In this work, we employed an approach to disentangle noncovalent and hydrogen-bonding electric field changes during the reaction cascade of a multidomain protein, i.e., the phytochrome Agp2. Agp2 originates from Agrobacterium fabrum and carries a biliverdin (BV) chromophore. Phytochromes harbor a methine-bridged tetrapyrrole chromophore as a light-sensing unit, which upon light absorption undergoes a photoisomerization at the terminal methine bridge followed by a cascade of structural relaxations.18−21 This reaction sequence interconverts the parent states Pr and Pfr and involves proton translocation, which has been shown to be a prerequisite for the functional secondary structure transition of the tongue, a phytochrome-specific peptide segment. In the present work, we have generated two further variants with ortho-cyanophenylalanine (oCNF) at positions 165 or 192.

We determined the crystal structures of the Pfr state of Y165oCNF and F192oCNF variants with 1.90 and 2.06 Å resolution, respectively. Structural details of the ZZEssa chromophore geometry and rotamer positions of amino acids within the CBP display a very high similarity between the oCNF variants and the WT protein, whereby F192oCNF is virtually indistinguishable from the WT. The region between 1500 and 1700 cm–1 is dominated by the C=C stretching modes of the methine bridges between pyrrole rings, which are particularly sensitive toward geometrical changes of the tetrapyrrole skeleton.54 In the Pfr state, a nearly perfect agreement between the WT and F192oCNF spectra in this region underpins the preservation of the chromophore structure in both proteins. In the Pr-minus-Pfr difference spectrum of F192oCNF, the lack of a positive band in this region confirms the shift of the tautomeric equilibrium toward the enol form. Phe192 is located in a hydrophobic part of the CBP. Accordingly, no strong H-bonds are expected for either pCNF or oCNF at position 192, which is confirmed by the crystal structure (F192oCNF) and the structural model (F192pCNF) for the Pfr state with the exception of a H-bond in the oCNF192 backbone to Gly173. For the sake of simplicity, we may therefore classify the H-bonds of the protein-bound phenyl substituents on the basis of the EF,tot,HB values as very weak (0–15 MV/cm), weak (15–30 MV/cm), medium (30–45 MV/cm), strong (45–60 MV/cm), and very strong (>60 MV/cm). Both F192pCNF and F192oCNF reveal only very weak H-bonding interactions because this residue is located in an essentially nonpolar pocket as shown by Pfr structures. A strong field increase upon Pr formation is also found for F192pCNF and F192oCNF, which is, however, accompanied by minima in Lumi-F and Meta-F, respectively. In both Agp2 variants carrying the nitrile group at the ortho position, the noncovalent electric fields remain largely constant during the photoconversion.

>[2x]MASTDYHVDLTNCDREPIHIPGYIQPHGCLIACDNAMRMVLRHSENCGELLGLEGDLNGRTAEDVLGKKLVHDLRNALTVTGRTTRPAMLPAMETSDGRSFDISLHRYKSTTIIEFEPSGSDAQPLGTARKMVDRIREADSVESLISRTTRLVKATLGYDRVMIYRFQEDGAGKVVSEAKQPELESFLGQYXPASDIPQQARALYLKNTLRIISDASGTRIPVLPAVDVSGEPLDLSYAHLRSVSPIHCEYLRNMGVAASMSISVIVDGALWGLIACHHYSPRVLSMPVRIAAEMFGEFFSMHLQVLKQKRRLDTINHAHAALDRFLRLAAHHANIEELLVDSFQDFADLMPCDGVGLWVGNNWHGHGATPPHDAIPRLARFVASASEGRVWATHALSQAIPEAEIYAGTAAGMLAIPLSQVKSDYLLFFRKEIVQNLNWAGNPEKSYETGPMGDRLTPRKSFAIWKETVRLQAQPWSEADREIAEAARIALVEVAFHHSEHHHHHH> SGTFFKDYQ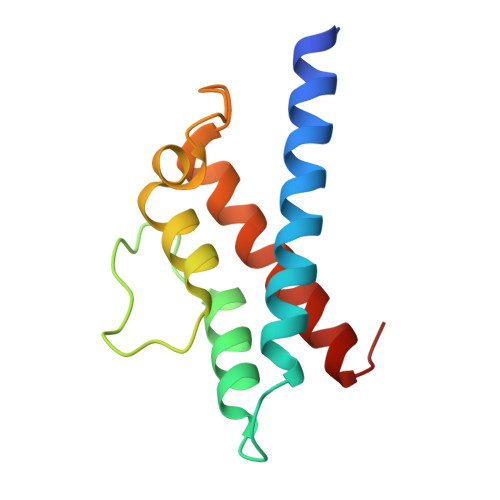KKNVMRLLQDSLEKIINEWLKTDDESHTKLKSLQELSEMDINATSFAEHSPLPDFVTRLWLDPHKALDAMDKNISKNEIRKLIKETAREIELVFTHQK> MRGSHHHHHHGSKDSTVQTSISVENVLERAGDSTPFSIALESIDAMKTIEEITIAGSGKASFSPLTFTTVGQYTYRVYQKPSQNKDYQADTTVFDVLVYVTYDEDGTLVAK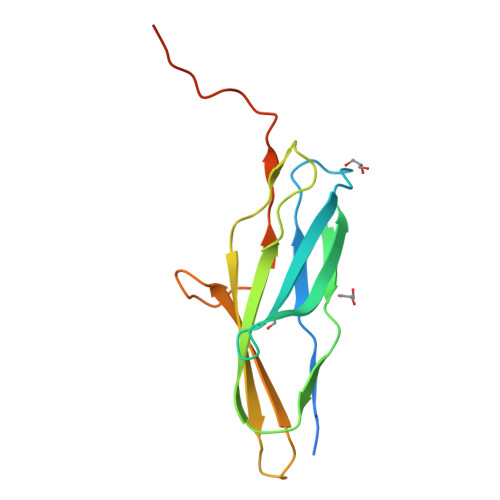VISRRAGDEEKSAITFKPKWLVKPIPPRQPNIPKTPLPLA>[4x]MGSSHHHHHHSSGRENLYFQGITEKNMKLSEGAYRAKLADMVGNYKDVIKVLTESSDFRDNSLILLLAGSLRNRVTSIRNSLKSIKSQEEKLRKEKSLNNEFIQVIEDIKRDFEESILLESEDVIRIIDDNLLMYSEEGARAFCIKLKGDLMRYKAEILKDEEKNQCIKQAVEFYEDALQRERSFLEKYPSDPLYLATI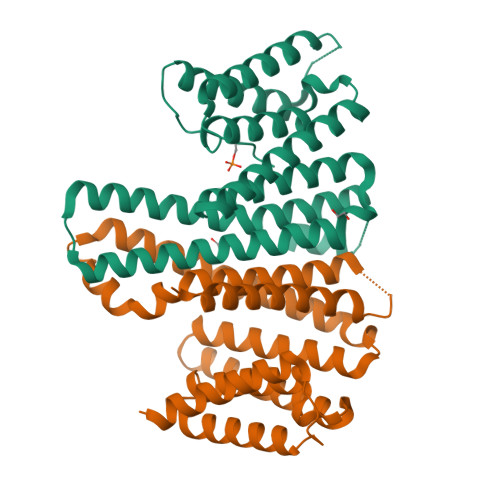LNYTILKYDLLGNPEGAMKFANRAIQAAENSRSDSEQFSENTEKLLKILRDNVSQWEQGCSGLLTSAFF>[3x]HMDDISQDNFLLSKEYENSLDVDTKKASGIYYTPKIIVDYIVKKTLKNHDIIKNPYPRILDISCGCGNFLLEVYDILYDLFEENIYELKKKYDENYWTVDNIHRHILNYCIYGADIDEKAISILKDSLTNKKVVNDLDESDIKINLFCCDSLKKKWRYKFDYIVGNPPYIGHKKLEKKYKKFLLEKYSEVYKDKADLYFCFYKKIIDILKQGGIGSVITPRYFLESLSG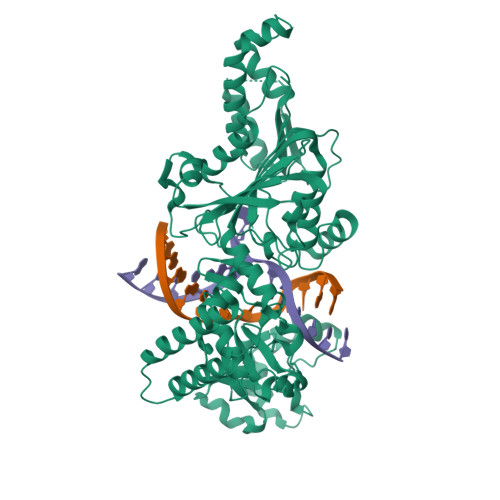KDLREYIKSNVNVQEIVDFLGANIFKNIGVSSCILTFDKKKTKETYIDVFKIKNEDICINKFETLEELLKSSKFEHFNINQRLLSDEWILVNKDDETFYNKIQEKCKYSLEDIAISFQGIITGCDKAFILSKDDVKLNLVDDKFLKCWIKSKNINKYIVDKSEYRLIYSNDIDNENTNKRILDEIIGLYKTKLENRRECKSGIRKWYELQWGREKLFFERKKIMYPYKSNENRFAIDYDNNFSSADVYSFFIKEEYLDKFSYEYLVGILNSSVYDKYFKITAKKMSKNIYDYYPNKVMKIRIFRDNNYEEIENLSKQIISILLNKSIDKGKVEKLQIKMDNLIMDSLGI>LPNITILATGGTIAGGGDSATKSNYTVGKVGVENLVNAVPQLKDIANVKGEQVVNIGSQDMNDNVWLTLAKKINTDCDKTDGFVITHGTETMEETAYFLDLTVKCDKPVVMVGAMRPSTSMSADGPFNLYNAVVTAADKASANRGVLVVMNDTVLDGRDVTKTNTTDVATFKSVNYGPLGYIHNGKIDYQRTPARKHTSDTPFDVSKLNELPKVGIVYNYANASDLPAKALVDAGYDGIVSAGVGNGNLYKSVFD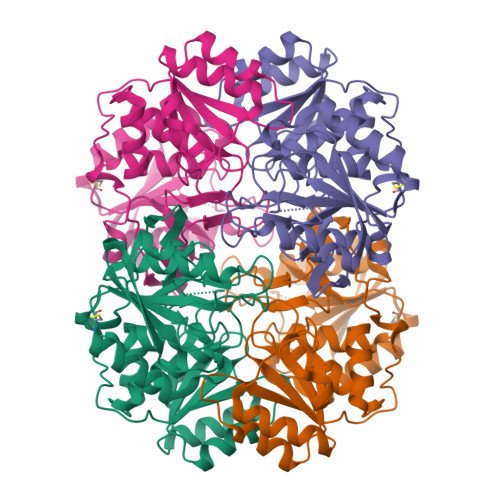TLATAAKTGTAVVRSSRVPTGATTQDAEVDDAKYGFVASGTLNPQKARVLLQLALTQTKDPQQIQQIFNQY[2x]>MSTFEDADEEETVTCLQMTIYHPGQQSGIFKSIRFSSKEKFPSIEVVKFGRNSNMCQYTFQDKQVSRIQFVLQPFKQFNSSVLSFE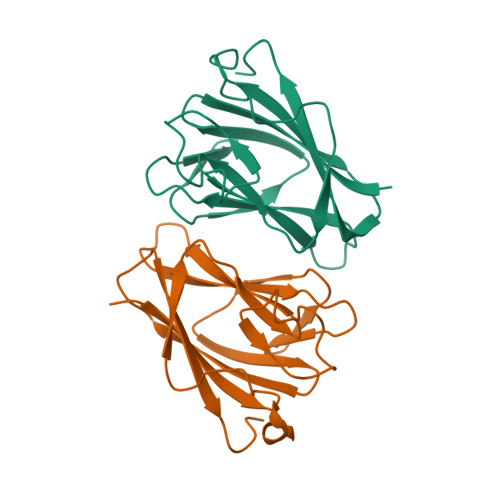IKNMSKKTSLMVDNQELGYLNKMDLPYKCMLRFGEYQFLLQKEDGESVESFETQFIMSSRPLLQENNWPTQNPIPEDGMYSSYFTHRSSPSEMDENELLEHHHHHH[6x]> GSGAKSLFSTAFSESLAAEISSVSRDELMEAIQ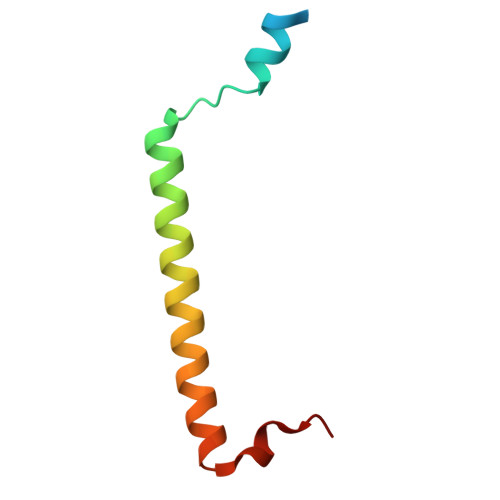KQEEINFRLQDYIDRIIVAIMETNPSILEVK9-(2-DEOXY-BETA-D-RIBOFURANOSYL)-6-METHYLPURINE | 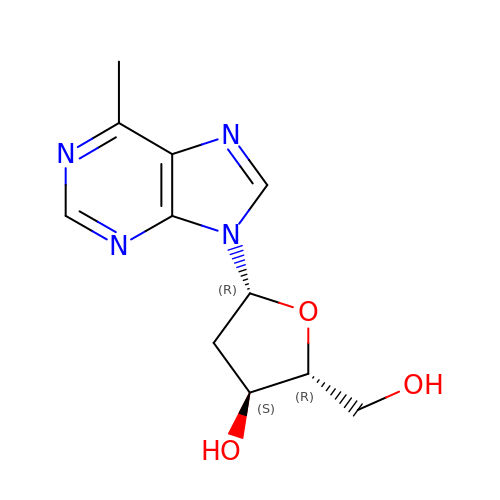C11 H14 N4 O3 | SJXRKKYXNZWKDB-DJLDLDEBSA-N>[14x]MSSERTFIAVKPDGVQRGLVGEIIARFERKGYKLVALKILQPTTE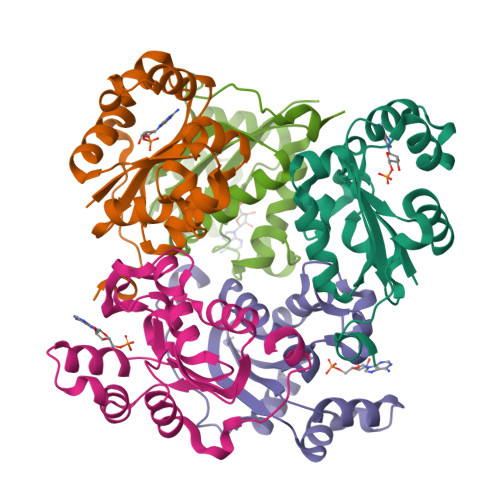QAQGHYKDLCSKPFFPALVKYFSSGPIVCMVWEGKNVVKSGRVLLGATNPADSQPGTIRGDFAVDVGRNVCHGSDSVESAEREIAFWFKADEIASWTSHSVSQIYE>HHHHHHFNLPPGNYKKPKLLYCSNGGH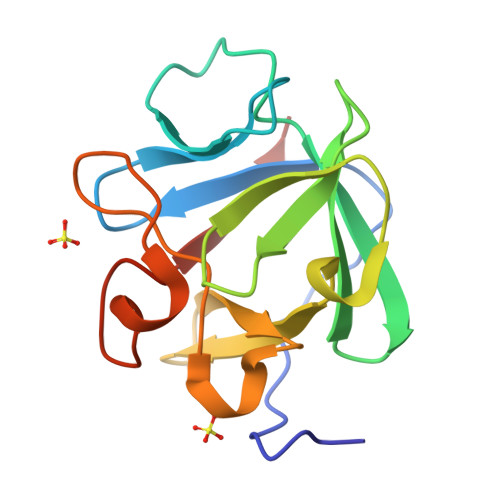FLRILPDGTVDGTRDRSDQHIQLQLSAESVGEVYIKSTETGQYLAMDTDGLVYGSQTPNEECLFLERLEENHYNTYISKKHAEKNWFVGLKKNGSCKRGPRTHYGQKAILFLPLPVSSD[2x]>MAHHHHHHMQHPTSTDIQRVREFLLDLQARICAGLEQQEKAGGGTAEFIIDDWERPEGGGGRSRVLQNGTVIEKGGVMFSHINISKLPASATERHPQIAGAKAQALGVSLVIHPKNPNIPTSHANVRLFVAEREDQDPIWWFGGGFDLTPFYPDDQDVLNWHQAAYDLCKPFGDNVYAEHKKWCDDYFYLKHRDEQRGVGGLFFDDLNCWDFETCFKYIQAVGNGYLNAILPIFEKHREQPYTEAQREFQLYRRGRYVEYNL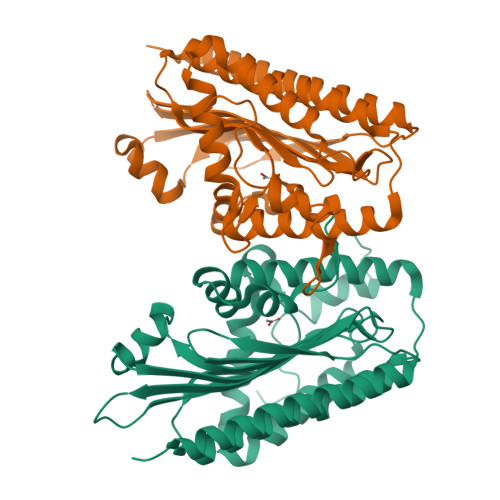VYDRGTLFGLQTGGRIESILVSLPNLAAWSYRPEWDEDSPEKRLTDYYLKPRDWLGLEEKVA[2x]>MDIGDNSKFDSATDLPVEQEQEQETEQEGEPEESSEQDLVEEVDWKDIPVPADAGPNMKWEFQEISDNFEYEAPADNKGSEFLEKWDDFYHNAWAGPGLTEWKRDRSYVADGELKMWATRKPGSDKINMGCITSKTRVVYPVYIEARAKVMNSTLASDVWLLSADDTQEIDILEAYGADYSESAGKDHSYFSKKVHISHHVFIRDPFQDYQPKDAGSWFEDGTVWNKEFHRFGVYWRDPWHLEYYIDGVLVRTVSGKDIIDPKHFTNTTDPGNTEIDTRTGLNKEMDIIINTEDQTWRSSPASGLQSNTYTPTDNELSNIENNTFGVDWIRIYK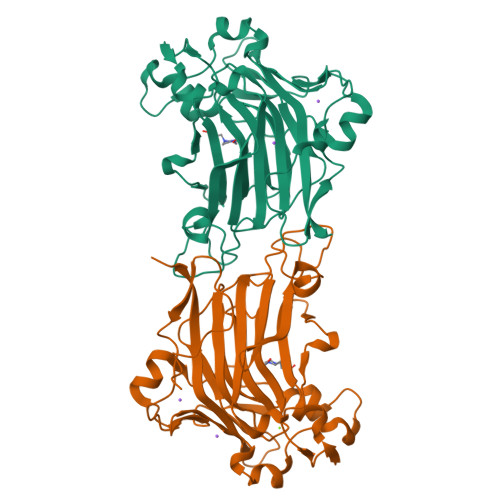PVEKLEHHHHHH[4x]> GLDVAISQNGFFRLVDSNGSVFYSRNGQFKLDENRNLVNMQGMQLTGYPATGTPPTIQQGANPAPITIPNTLMAAKSTTTASMQINLNSTDPVPSKTPFSVSDADSYNKKGTVTVYDSQGNAHDMNVYFVKTKDNEWAVYTHDSSDPAATAPTTASTTLKFNENGILESGGTVNITTGTINGATA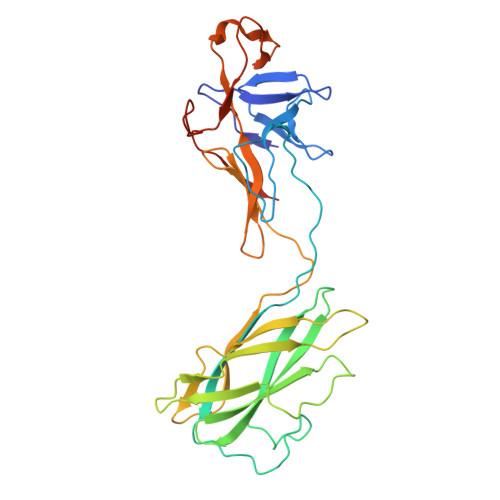ATFSLSFLNSMQQNTGANNIVATNQNGYKPGDLVSYQINNDGTVVGNYSNEQEQVLGQIVLANFANNEGLASQGDNVWAATQASGVALLGTAGSGNFGKLTNGALEASNVDLSK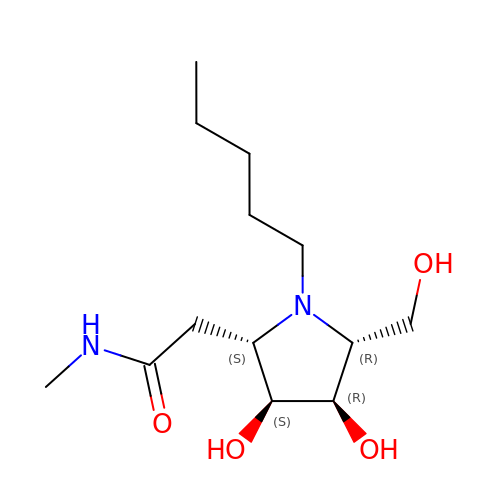2-[(2S,3S,4R,5R)-5-(hydroxymethyl)-3,4-bis(oxidanyl)-1-pentyl-pyrrolidin-2-yl]-N-methyl-ethanamide | C13 H26 N2 O4 | NZYWNYJYZSBEBH-JULQROHOSA-N> MTSSTQEPLNA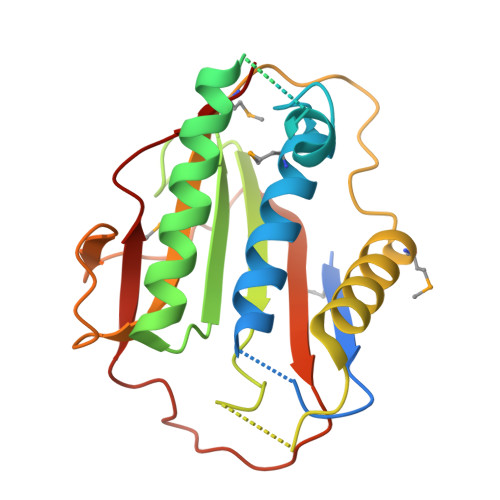SEAFCPRDCMVPVVFPGPVSQEGCCQFTCELLKHIMYQRQQLPLPYEQLKHFYRKPSPQAEEMLKKKPRATTEVSSRKCQQALAELESVLSHLEDFFARTLVPRVLILLGGNALSPKEFYELDLSLLAPYSVDQSLSTAACLRRLFRAIFMADAFSELQAPPLMGTVVMAQGHRNCGEDWFRPKLNYRVPSRGHKLTVTLSCGRPSIRTTAWEDYIWFQAPVTFKGFRE N-{(3R)-1-[3-(propan-2-yl)-1H-pyrazole-5-carbonyl]pyrrolidin-3-yl}cyclopropanecarboxamide 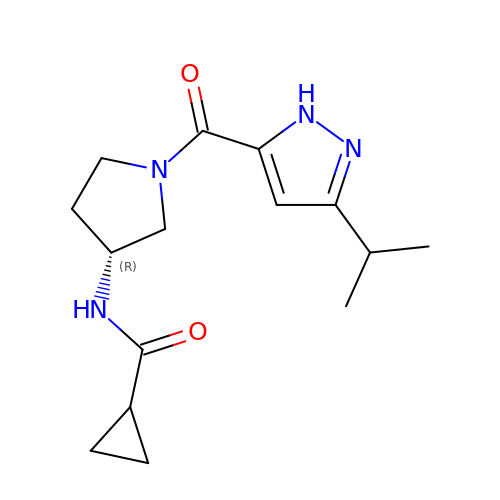| C15 H22 N4 O2 | CXEXTVGTDZRKJS-LLVKDONJSA-N> ETGGLLNCP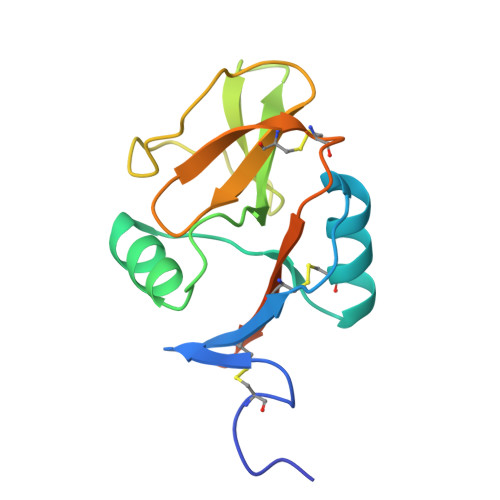IYWQQLREKCLLFSHTVNPWNNSLADCSTKESSLLLIRDKDELIHTQNLIRDKAILFWIGLNFSLSEKNWKWINGSFLNSNDLEIRGDAKENSCISISQTSVYSEYCSTEIRWICQKELTPVRNKVYPDSKHHHHHH> MGSSFEVIARTAYEEGRTRLATELLNHEPRAGRQVPLLLSMEEDELALDKAIESGDTDLIYFVIHQLRRKLPLASFFRVVSSRPTASAMVEALARNSDGDGNEDTALLKDLYYQDDRRLDGASVFIREALQQPETRTASDKLDLA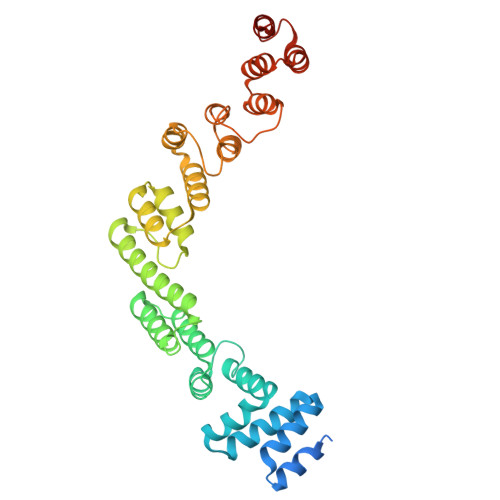ANLLQGNQKEHVFELGALKEAKMLLRMQETFERDLTDSFVGLSVNQTMFKLIKLGYHGRAKKIQSEFKVPERVAWWIRLQALVAKRDWNEIEEISRQRKSPIGWEPFFNQVLQAGNPRLAATFIPKCTNLEPGQTITMYEKCGMRVKAAEEAVRLKDTEAWNRLLEAAGRNTAEGREIERLGATVFKK>[4x]GSYDKVSQAKSIIIGTKQTVKALKRGSVKEVVVAKDAD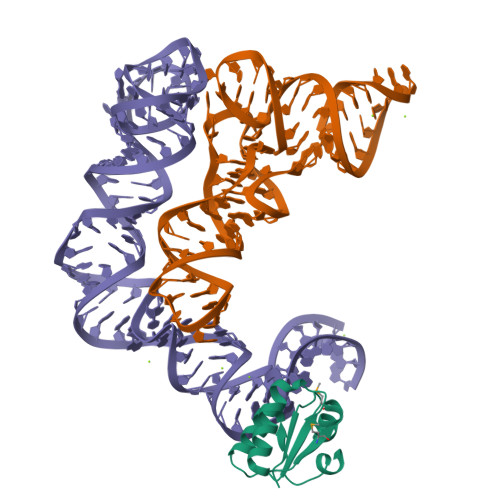PILTSSVVSLAEDQGISVSMVESMKKLGKACGIEVGAAAVAIIL> GPGADRAQDHNNNNTPRNSNYVVEEEEVSEEEEEAIMMPDFGDHVDTSIFGQILEMDEGDDHDFSAPLVLNFFEQAEETFQKMETALNNKDLPELSKLGEFLKGSSATLGFTKIRDSCQLIQQYGHGLNVDGSSEPDEGVCLKKIAEALASARVDTVALHKMMREFFEY

If the HK incorporates a REC domain (REC-1) is denoted as hybrid histidine kinase (hHK), and the first His-Asp phosphotransfer event occurs in the same polypeptide chain. Then, HPt protein containing a phosphorylatable His shuffles the phosphoryl group from the phosphorylatable Asp in the REC-1 domain to the phosphorylatable Asp in the REC domain of an RR (REC-2) in two more phosphotransfer steps. In fungi, the HPt accepts the phosphoryl group from REC-1 domains of various hHKs upstream of the signaling pathway and forwards it downstream to REC-2 domains present in at least two conserved RRs, Ssk1 and Skn7. Also, we have obtained the crystal structures of Ct_HPt alone and in complex with REChHK6 bound to the phosphomimetic BeF3−, as well as the crystal structures of REChHK3 and RECCa_Sln1.

To assess that phosphotransfer from REC-1 domains was being carried out on the phosphorylatable H105 of Ct_HPt, we generated the mutant H105E and conducted phosphotransfer experiments with REChHK6 and REChHK3 in the presence of PAM. The absence of electrophoretic mobility shift for the Ct_HPt mutant H105E in the presence of PAM, compared to WT, alone or upon incubation with the REC-1 domains indicated the absence of phosphotransfer and confirmed H105 as the only nucleophilic residue to become phosphorylated. We determined the structure of the phosphomutant Ct_HPt H105E at 2.4 Å which showed a similar structure than Ct_HPt in the complex (rmsd of 0.7 Å for 125 residues). However, the superposition of the phosphomutant to the complex showed few clashes with residues of REChHK6 involved in complex interactions, thus, supporting that subtle changes in the side chain conformation of a few residues could prevent phosphotransfer. In relation to HPt, we have observed subtle changes in the phosphomimetic mutant H105E.Noroviruses are highly contagious, infecting both humans and animals. The human norovirus capsid protruding (P) domain binds histo-blood group antigen (HBGA) co-factors for infection, and a recently discovered bat norovirus (GX) was also found to interact with HBGAs. In this study, we determined the P domain structures of four human noroviruses and one bat norovirus using X-ray crystallography to examine structural features linked to potential interspecies transmission. The principal structural difference was a variable length P2 subdomain loop (Loop A), which was located near the HBGA pocket.

The P domains of GII.9 (AY038599), GII.23 (KT290889), GII.27 (MG495077), GVIII (AJ844470), and GX (MF373609) were expressed in E.coli. The five P domains were structurally equivalent with a root mean square deviation for C-alpha atoms ranging between 0.586 Å (GII.23-GII.27) and 1.645 Å (GII.9-GX). The cross-reactivity of the P domains was determined using direct ELISA with a broad-spectrum human norovirus Nanobody (Fc-NB26) that binds to a highly conserved region on the P domain. Fc-NB26 bound to GII.9, GII.23, and GII. P domains in a dose-dependent manner at concentrations less than 80 ng/mL. Structural modeling of the Fc-NB26-binding site indicated that GII.9, GII.23, and GII. P domains contained most of the equivalent residues that could interact with Fc-NB26. Our cumulative data show that Fc-NB26/NB26 binds most GII genotypes, and the epitope is vulnerable and a therapeutic target region for GII noroviruses.

>[2x]SKPFTIPILTIGEMTNSRFPVPIDMLHTSPTENIVVQPQNGRCTIDGELLGTTQLITSNICSFRGSISGHEGNDDQHLWHFNITNPNGTPFDPTEDVPAPLGTPDFRGQLYGVISQRDREGTPSENNQKANRSHQGVISTISPKFVPKLGSVMIGTWTTDDIKNQPSKFTPIGLNDDDNFKQWELPNYSGALTLNMGLAPSVFPTYPGEQILFFRSYLPLKGGYGSPFIDCLVPQEWVAHFYQESAPAQTDVALIRYVNPETGRVLFEAKLHRQGFITVAKSGDSPINVPANGYFRFDSWVNQFYSLAPM>MAQPIVFYDIPSNERIKHSPWSPNTWKIRYALNYKGLKYKTEWVEYPDIAGVVQKLGGKPTEKTPDGRDHYTLPVIYDPNTKKVVEDSAAIAKYLDETYPDTPKLFPAGTDAFQAAFLDFAWPVLGFPVFMLVILDTANSLLPRSHDYFRSTREQKFGKKLEELATEEEWAKVEAGLAKLKGYLDANGKGNDLLLMGAQGGITYSDIQIASFFVWAKIIWGEGSEKWKRLI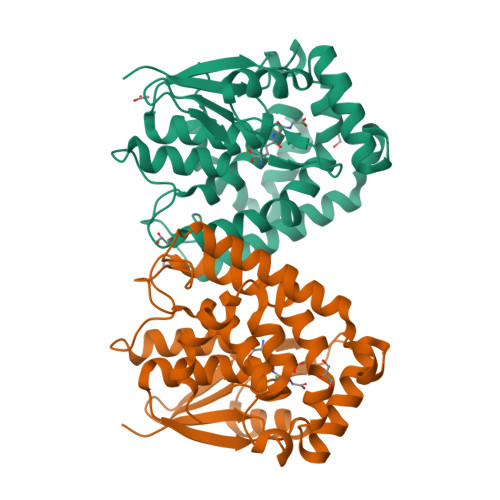SLHDGKWAQFYAQFTKFEQVDV[4x]dimethyl (2R)-5-(3-fluorophenyl)-1H-pyrrolo[1,2-c][1,3]thiazole-6,7-dicarboxylate 2-oxide | C16 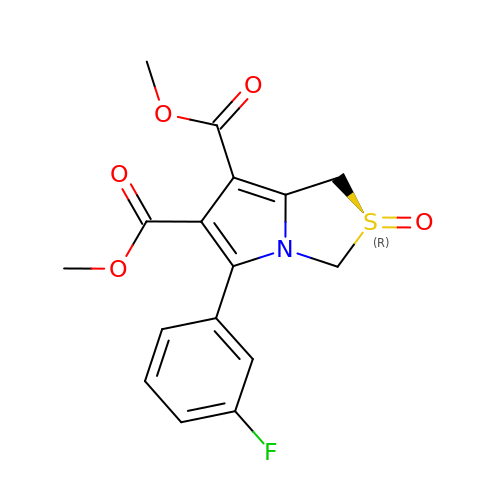H14 F N O5 S | KCIMLJNZZQRAFE-XMMPIXPASA-N> GPGYQDPNSAKLLQILNVRVVGSGERVVVLSHGFGTDQSAWSRVLPYLTRDHRVVLYDLVCAGSVNPDHFDFRRYDNLDAYVDDLLAILDALRIPRCAFVGHSVSAMIGILASIRRPDLFAKLVLIGASPRFLNDSDYHGGFELEEIQQVFDAMGANYSAWATGYAPLAVGADVPAAVQEFSRTLFNMRPDISLHVCQTVFKTDLRGVLGMVRAPCVVVQTTRDVSVPASVAAYLKAHLGG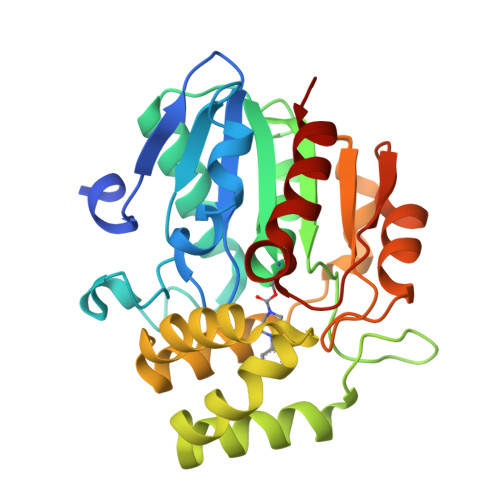RTTVEFLQTEGHLPHLSAPSLLAQVLRRALARY>[3x]MTPASYNLAVRRAAPAVVNVYNRGLNTNSHNQLEIRTLGSGVIMDQRGYIITNKHVINDADQIIVALQDGRVFEALLVGSDSLTDLAVLKINATGGLPTIPINARRVPHIGDVVLAIGNPYNLGQTITQGIISATGRIGLNPTGRQNFLQTDASINHGNSGGALVNSLGELMGINTLSFDKSNDGETPE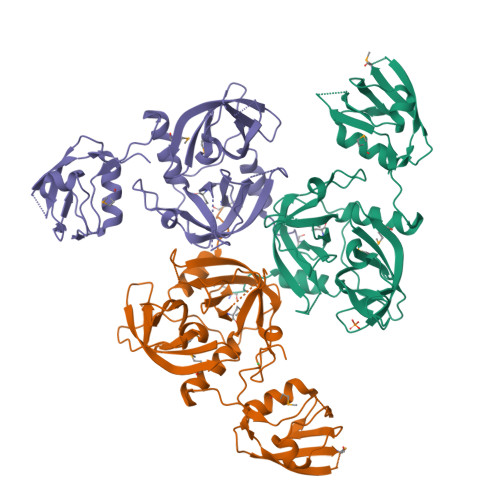GIGFAIPFQLATKIMDKLIRDGRVIRGYIGIGGREIAPLHAQGGGIDQLQGIVVNEVSPDGPAANAGIQVNDLIISVDNKPAISALETMDQVAEIRPGSVIPVVVMRDDKQLTLQVTIQEYPATNHHHHHH>[2x]MEAVKTFNSELYSLNDYKPPISKAKMTQITKAAIKAIKFYKHVVQSVEKFIQKCKPEYKVPGLYVIDSIVRQSRHQFG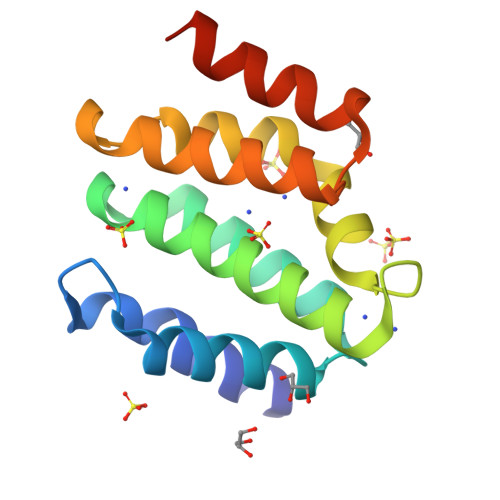QEKDVFAPRFSNNIISTFQNLYRCPGDDKSKIVRVLNLWQKNNVFKSEIIQPLLDMAAALEHHHHHH>MIGILGGGQLGRMLALAGYPLGLSFRFLDPSPEACAGQVGELVVGEFLDEGALLRFAEGLALVTYEFENVPVEAARRLEGRLPLYPPAKALEVAQDRLREKTFFQGLGVPTPPFHPVDGPEDLEEGLKRVGLPALLKTRRGGYDGKGQALVRTEEEALEALKALGGRGLILEGFVPFDREVSLLAVRGRTGEVAFYPLVENRHWGGILRLSLAPAPGASEALQKKAEAYALRAMEALDYVGVLALEFFQVGEELLFNEMAPRVHNSGHWTIEGAETSQFENHLRAVLGLPLGSTAPRGQSAMVNLIGEK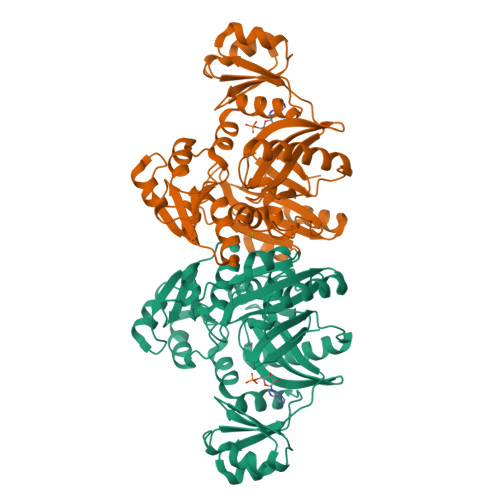PPFAEVLKVEGAHLHWYGKAVRPGRKVGHITLRRDGLKALEEGLARLSRLVSELPWEGRV[2x]> PTEFLYTSKIAAISWAATGGRQQRVYFQDLNGKIREAQRGGDNPWTGGSSQNVIGEAKLFSPLAAVTWKSAQGIQIRVYCVNKDNILSEFVYDGSKWITGQLGSVGVKVGSNSKLAALQWGGSESAPPNIRVYYQKSNGSGS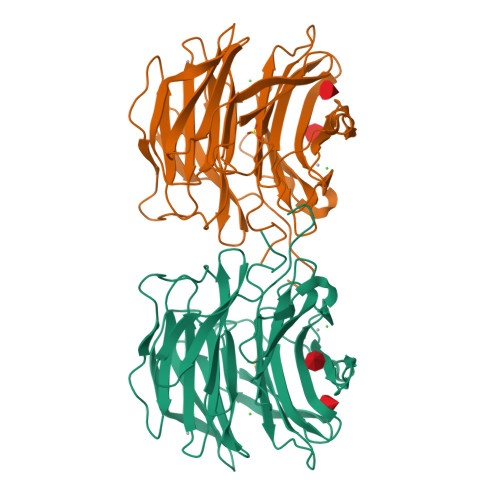SIHEYVWSGKWTAGASFGSTVPGTGIGATAIGPGRLRIYYQATDNKIREHCWDSNSWYVGGFSASASAGVSIAAISWGSTPNIRVYWQKGREELYEAAYGGSWNTPGQIKDASRPTPSLPDTFIAANSSGNIDISVFFQASGVSLQQWQWISGKGWSIGAVVPTGTPAGW>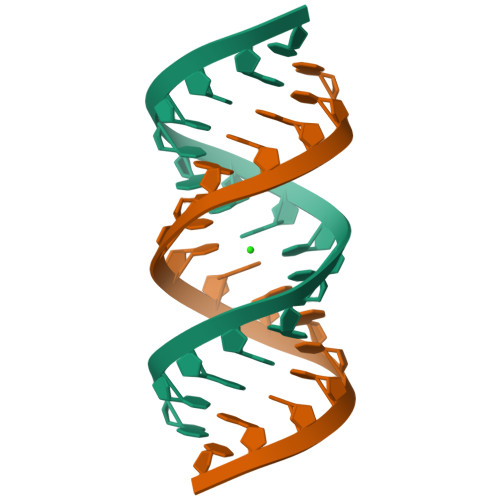GCAGACUUAAAUCUGC[3x]2-amino-1-[(3S)-3-methyl-4-(4-methylisoquinoline-5-sulfonyl)-1,4-diazepan-1-yl]ethan-1-one 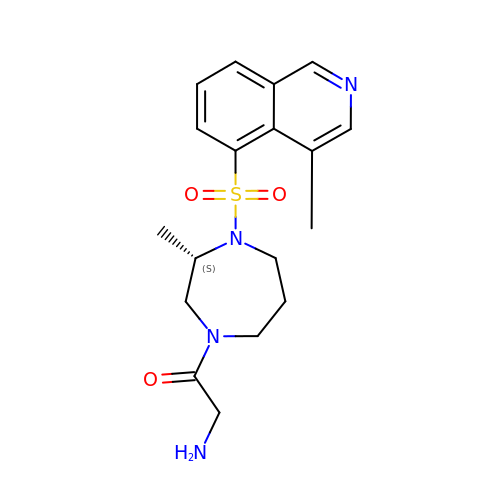| C18 H24 N4 O3 S | CMKMGFAUKPAOMG-AWEZNQCLSA-N>MPVGFIGLGNMGNPMAKNLMKHGYPLIIYDVFPDACKEFQDAGEQVVSSPADVAEKADRIITMLPTSINAIEAYSGANGILKKVKKGSLLIDSSTIDPAVSKELAKEVEKMGAVFMDAPVSGGVGAARSGNLTFMVGGVEDEFAAAQELLGCMGSNVVYCGAVGTGQAAKICNNMLLAISMIGTAEAMNLGIRLGLDPKLLAKILNMSSGRCWSSDTYNPVPGVMDGVPSANNYQGGFGTTLMAKDLGLAQDSATSTKSPILLGSLAHQIYR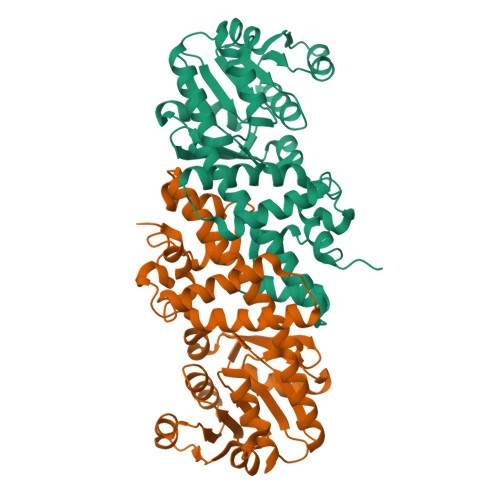MMCAKGYSKKDFSSVFQFLREEET[4x]>MVSLLRRTFSEEIKEELVNVPFGSREEVISELLGFIKARGDLDVKSRHIVFSLHSFAASRRLLNLMKYLSKPVSEIIVEKSHNIKKRYIKITAEYSESFMVIEPFFDVALFVSFLRGLFLSGGSMTN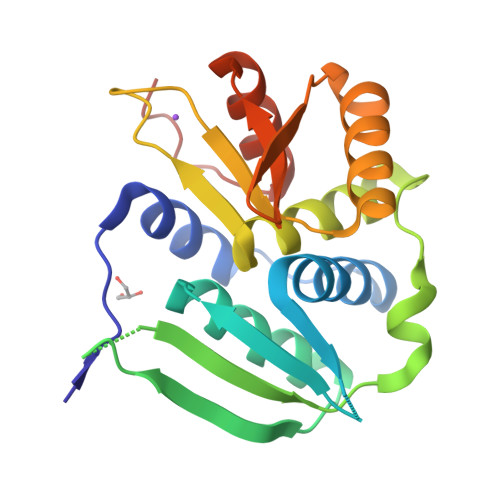PRYHYHLEINLFEEETLALTRKSLKDFFNINAGIIELRNTRKLYIKSIKDILVFLEAIGVQRKLEEIDRIV[2x]>[3x]MAEQLVEAPAYARTLDRAVEYLLSCQKDEGYWWGPLLSNVTMEAEYVLLCHILDRVDRDRMEKIRRYLLHEQREDGTWALYPGGPPDLDTTIEAYVALKYIGMSRDEEPMQKALRFIQSQGGIESSRVFTRMWLALVGEYPWEKVPMVPPEIMFLGKRM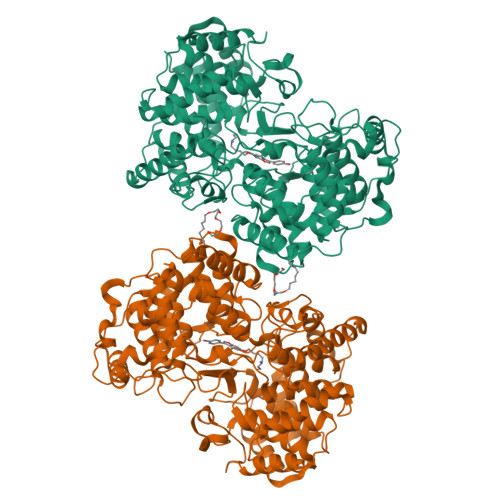PLNIYEFGSWARATVVALSIVMSRQPVFPLPERARVPELYETDVPPRRRGAKGGGGWIFDALDRALHGYQKLSVHPFRRAAEIRALDWLLERQAGDGSWGGIQPPWFYALIALKILDMTQHPAFIKGWEGLELYGVELDYGGWMFQASISPVWDTGLAVLALRAAGLPADHDRLVKAGEWLLDRQITVPGDWAVKRPNLKPGGFAFQFDNVYYPDVDDTAVVVWALNTLRLPDERRRRDAMTKGFRWIVGMQSSNGGWGAYDVDNTSDLPNHIPFCDFGEVTDPPSEDVTAHVLECFGSFGYDDAWKVIRRAVEYLKREQKPDGSWFGRWGVNYLYGTGAVVSALKAVGIDTREPYIQKALDWVEQHQNPDGGWGEDCRSYEDPAYAGKGASTPSQTAWALMALIAGGRAESEAARRGVQYLVETQRPDGGWDEPYYTGTGFPGDFYLGYTMYRHVFPTLALGRYKQAIERR The lysine-biosynthesis pathway commences with the condensation of pyruvate and (S)-aspartate semialdehyde (ASA), to form (4S)-4-hydroxy-2,3,4,5-tetrahydro-(2S)-dipicolinic acid (HTPA). This reaction is catalyzed by dihydrodipicolinate synthase (DHDPS), which is the product of an essential gene in bacteria. The ‘tight’ dimer interface also contains a cleft that binds the allosteric inhibitor, lysine, which mediates feedback inhibition in DHDPS enzymes from Gram-negative bacteria and plants. In this study, we show for the first time that DHDPS from the plant Vitis vinifera forms a homotetramer or dimer-of-dimers both in solution and the crystal state.

The asymmetric unit contains two tetramers comprised of four identical subunits. Each tetramer can be described as a dimer-of-dimers, with the monomers within the two dimeric units ab and cd tightly bound to each other, and weaker interactions between monomers ac and bd. The quaternary architecture of the Vv-DHDPS tetramer is identical to the N. sylvestris structure and quite distinctive from the typical bacterial tetramer. Each monomer comprises an N-terminal (β/α)8-barrel domain and a C-terminal domain consisting of 3 α-helices and 2 short β-strands. The active site centers around Lys184, which forms a Schiff base with pyruvate and is located at the center of each monomeric unit. Three hydroxyl-containing amino acids, namely Tyr132, Thr69 and Tyr156, form the conserved catalytic triad with Tyr132 contributed from the adjacent monomer across the ‘tight’ dimer interface (i.e. interface between subunits ab or cd). Examination of potential interfaces within the enzyme using the Protein Interfaces, Surfaces and Assemblies (PISA) program show that each of the two tight dimer interfaces (ab and cd) bury approximately 1790 Å2 per monomer, which corresponds to ∼14% of the total surface area of the monomer. By contrast, the interfaces between monomers a & c and b & d, bury a surface area of approximately 630 Å2 per monomer. In addition, the lack of electron density observed for the N-terminal region (including the His-tag) indicates that this region is highly flexible. The larger RMSFs observed for the dimer include the key catalytic residues Thr69, Tyr156 and Lys184, as well as Tyr132, which interdigitates across the ‘tight’ dimer interface to form part of the active site of the adjacent monomer. These data suggest that the dimer possesses greater conformational flexibility than the wild-type tetramer, and thus formation of the ‘back-to-back’ dimer-of-dimers functions to attenuate protein dynamics.

>[8x]MGSSHHHHHSSGLVPRGSHMAVIPNFHLPMRSFEVKNRTSVDDIKSLRLITAIKTPYLPDGRFDLEAYDALVNMQIVDGAEGVIVGGTTGEGQLMSWDEHIMLIGHTVNCFGGSIKVIGNTGSNSTREAIHATEQGFAVGMHAALHINPYYGKTSLEGLVSHFESVLPMGPTVIYNVPSRTGQDIPPGVIHTVAQSANLAGVKECVGNDRIKQYTDNRIVVWSGNDDQCHDAKWDYGATGVISVTSNLIPGLMRQLLFKGKNPSLNAKIMPLVNWLFEEPNPIGLNTALAQLGVVRPVFRLPYVPLPLAKRVEFVNIVKEIGRENFVGEKDVKVLDDDDFILVGRY> GAMSSKNEWRKSAIANTLLYLRLKN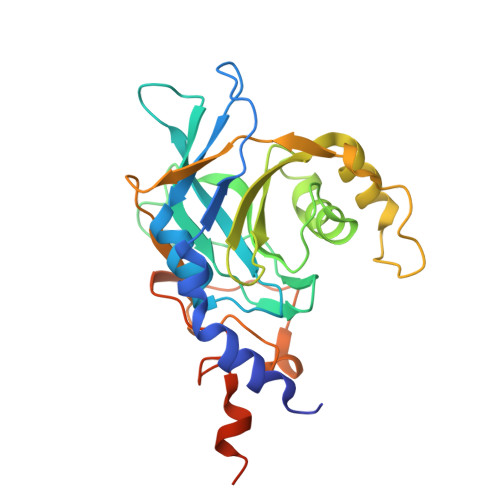IYVSADDFVEEQNVYVLPKNLLKKFIEISDVKIQVAAFIYGMSAKDHPKVKEIKTVVLVPQLGHVGSVQISNIPDIGDLPDTEGLELLGWIHTQTEELKFMAASEVATHSKLFADKKRDCIDISIFSTPGSVSLSAYNLTDEGYQWGEENKDIMNVLSEGFEPTFSTHAQLLLSDRITGNFIIPSGNVWNYTFMGTAFNQEGDYNFKYGIPLEFYNEMHRPVHFLQFSELAGDEELEAEQIDVFS>HHHHHHENLYFQGMEKVTVTLDERSYPINIAPSLYQQQDAFWPLTAGQRAMIVTNETLAPLYLHKIQTVLEVSGVKVDSIILPDGEQYKSLFIMNDVFTALLEKHHNRDTTLIALGGGVIGDLTGFAAASYQRGVRFIQVPTTLLSQVDSSVGGKTAVNHPLGKNMIGAFYQPASVVIDLDCLKTLPKRELSSGLAEVIKYGII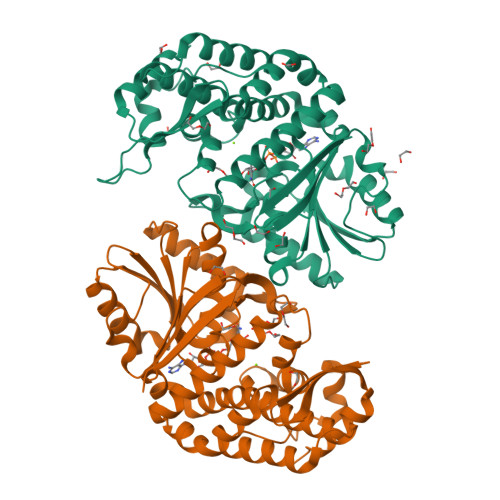LDGEFFSWLEENIDALMALDNQAMAYCIRRCCELKAQVVAADEKETSGLRALLNLGHTFGHAIEAEMGYGVWLHGEAVAAGMVMAAKTAELIGQFTPEQTDRVIALLKRAELPVTGPAKMQPDDYLPHMMRDKKVMGGKLHLILPTTIGHSEMRSDVDASTVTAAISACIP[4x]> GMDEQPLSRPGAHVKYAVLGATGLLGHHAARAIRAAGHDLVLIHRPSSQIQRLAYLEPECRVAEMLDHAGLERALRGLDGVIFSAGYYPSRPRRWQEEVASALGQTNPFYAACLQARVPRILYVGSAYAMP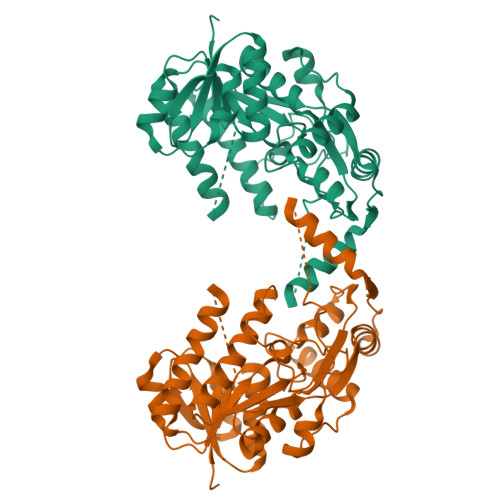RHPQGLPGHEGLFYDSLPSGKSSYVLCKWALDEQAREQARNGLPVVIGIPGMVLGELDIGPTTGRVITAIGNGEMTHYVAGQRNVIDAAEAGRGLLMALERGRIGERYLLTGHNLEMADLTRRIAELLGQPAPQPMSMAMARALATLGRLRYRVSGQLPLLDETAIEVMAGGQFLDGRKAREELGFFSTTALDDTLLRAIDWFRDNGYFNA(6~{S},9~{a}~{S})-6-(2-methylpropyl)-8-(naphthalen-1-ylmethyl)-4,7-bis(oxidanylidene)-~{N}-(phenylmethyl)-3,6,9,9~{a}-tetrahydro-2~{H}-pyrazino[1,2-a]pyrimidine-1-carboxamide | 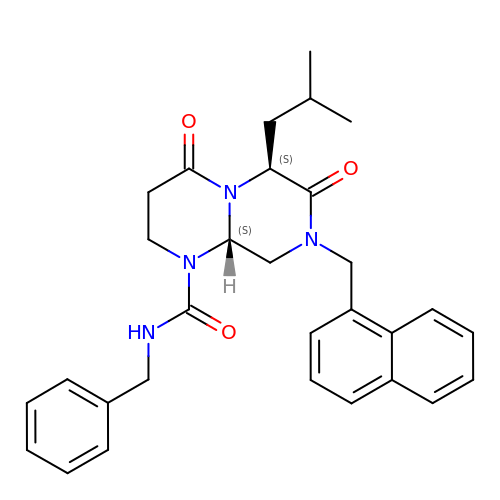C30 H34 N4 O3 | HABVPTFNPWNZNJ-RRPNLBNLSA-N> GHMDFS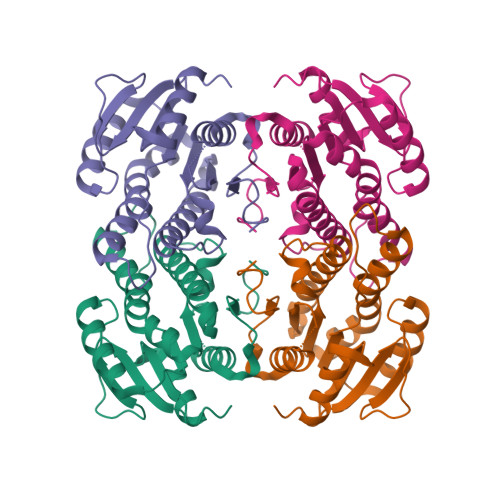GKNVWVTGAGKGIGYATALAFVEAGAKVTGFDQAFTQEQYPFATEVMDVADAAQVAQVCQRLLAETERLDALVNAAGILRMGATDQLSKEDWQQTFAVNVGGAFNLFQQTMNQFRRQRGGAIVTVASDAAHTPRIGMSAYGASKAALKSLALSVGLELAGSGVRCNVVSPGSTDTDMQRTLWVSDDAEEQRIRGFGEQFKLGIPLGKIARPQEIANTILFLASDLASHITLQDIVVDGGSTLGA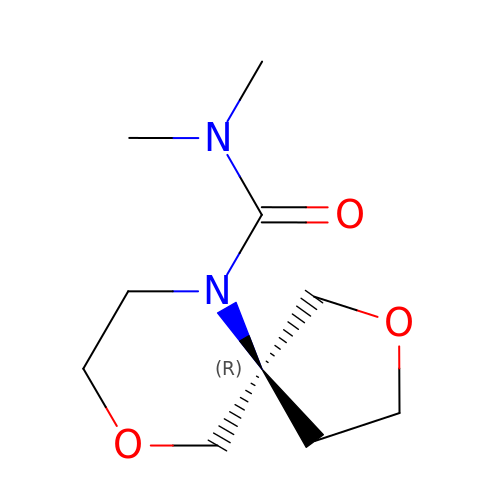(5R)-N,N-dimethyl-2,9-dioxa-6-azaspiro[4.5]decane-6-carboxamide | C10 H18 N2 O3 | RZCFMNWZMOAPRJ-SNVBAGLBSA-N> MRPRRRGLAYHHTKPKGQLSQGHYPTTSNDGQRRKVGNSEAFQSFDIWKNLDRIRSTKKNAGQFIKGSLLILPMRTEDKQQFDECMDELHKYISKDILRCYPQKEQKDEGMLFYIVLKDFNILDSCFVLSVLLAFQKRLWMAPSEKSYFRVPKNINLTGSFYLPKNIETGRGHIITSYRREQPSSSIVEVGFNVVPDFQQFQVKACHVSKFMNELSNFFSQVEFGKCEANVINYFKREYNRTYSQISLALYELPLIGDGLFDIKSYISKTRPIIETSKAQMIKHISEMKAYNEISGLQGDQFPRQQRPLSNSPSSNSISSSQTIEAGATSYQTQPQRHAVNKPSNVLNSSNRH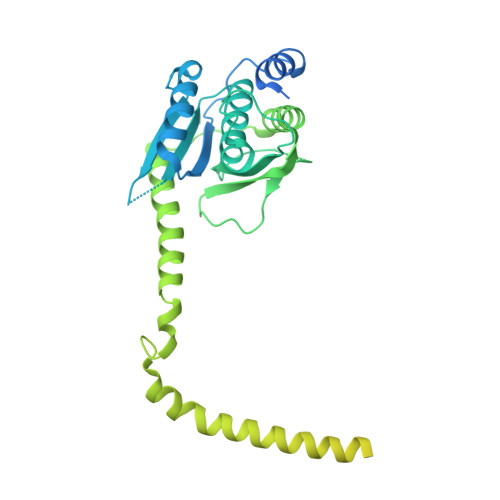SGPKTFEDGRYSEGNKPGFMTQDEIKQHCIGTIKASMDAVKKKSSYQILKTYVRCPRQNYIDIVYQNLNDLRSKTNCNIVVLNLNNLHESQMWLESLNTTNYTIFAQAPHPSTIRVISIGGVGEYIVKALELILNILEH> MLPEFPKIAVVAGSEAESVFRVVDIGTGDVVYEGRLSDSVYDDASGDTVRHADFGEWKRPGSYSVTVGRSSSAPFRIGNDVYRAPLIQAARSYTLARAGVAIDDPVTGLRHDVGHAQDKQAMLFFEDPFHRQGDPIDVSGGWYDAGDYGKYVPTGAVAAAQLMLAWEMRPELWRSLSLSLPAGLSEPERRAGLPDLLVEIKYELDWLLRMQRPDGAVYLKVAGGAWPGYIRPEEDTADRYVFGLSTYGTAQFAGAAAMGARVYAPFLPDYARKLLDAAIRAQRYLEQHPDPEFRYDEGQNNGSGPYEKRTDREERFWAAAELLRTTDDARYDAYIREHFSDFLEGKTSAVFWGNTVLLGQWAYVNAERADADHKASVRASLTAYADELVRWASANGYRSVLRPTDYFWGSAREAMGRAQALLLADAVAPNRAYLETALDQAHWLFGRNAAGTSFMTGIGMHSPQKPHHRLVASTQTLIPGLVVGGPNAQGGDPIMDRLLRESDPRVFPAKAYVDDWEAYSVNEPAIDYTAPAVFVLTRFAEDRGSGENLYFQGWSHPQFEKNSAVDGSGHHHHHHHH

J30, an endoglucanase with activity against p-nitrophenyl cellobiose (pNPC), which produces cellobiose as its primary product, was identified and analyzed from metagenomic data originating from a switchgrass-adapted microbial community. Its likely source is the moderately thermophilic bacterium Thermobacillus composti KWC4, and its catalytic optimum is 50°C. It is annotated as a GH family 9 member consisting of an N-terminal Ig-like domain and a C-terminal catalytic domain. The predominant architectural element of the catalytic domain is an (α/α)6-barrel structure composed of 12 α-helices arranged in an alternating pattern as is typical within GH family 9 as well as other families.

The substrate-binding cleft assumes the shape of an open channel. The interface between the Ig-like domain and the catalytic domain is stabilized by hydrophobic interactions, a salt bridge between Asp47 and Lys510, and seven hydrogen bonds between Glu4 and Arg431, Ile8 and Arg447, Asp42 and Asn395, Ala44 and Ala509, Asp47 and Tyr397, and His51 and both Gly396 and Arg398. The highly conserved acidic side chains of Asp147 and Glu523 are directly involved in the enzymatic catalysis. Glu523 acts as a proton donor, while Asp147 deprotonates the depicted water molecule for its nucleophilic attack. The carbohydrate ring in the +1 position is stacked between the side chains of Trp226 and Tyr519. In contrast to its closest homologs, J30 does not contain bound Ca2+ ions. In J30, the side-chain amino group of Lys308 forms hydrogen bonds to the Gly353 O atom and the Glu313 and Glu314 carboxyl groups at precisely the same site. The absence of this strand, and the associated hydrogen bonds that would connect it to β-strands 1 and 7 (J30 numbering) as well as to the catalytic domain, may contribute to the lower thermal tolerance of J30.> MADFLNFPRQMLPFSKKTKQWRKDCLLWANQKTFFNYSLVRKSVIHKKINYDLLNGRLHMSDLELVLNPDGIKAAYIPDRLQHYPIMNSKLNVLRGEESKRVFDFKVVVTNPNAISEIEDNKKNELLQRLQEMITDTSISEDEYNIKLEKLNDYYTYEWQDIREVRANELLNHYIKEYDIPLIFNNGFMDAMTCGEEIYQCDIVGGEPVIERVNPLKIRIFKSGYSNKVEDADMIILEDYWSPGRVIDTYYDVLSPKDIKYIETMPDYIGQGAVDQMDNIDERYGFVNQNMIGDEITVRDGTYFFDPANLFTEGIANSLLPYDLAGNLRVLRLYWKSKRKILKVKSYDPETGEEEWNFYPENYVVNKEAGEEVQSFWVNEAWEGTMIGNEIFVNMRPRLIQYNRLNNPSRCHFGIVGSIYNLNDSRPFSLVDMMKPYNYLYDAIHDRLNKAIASNWGSILELDLSKVPKGWDVGKWMYYARVNHIAVIDSFKEGTIGASTGKLAGALNNAGKGMIETNIGNYIQQQINLLEFIKMEMADVAGISKQREGQISQRETVGGVERATLQSSHITEWLFTIHDDVKKRALECFLETAKVALKGRNKKFQYILSDTSTRVMEIDGDEFAEADYGLVVDNSNGTQELQQKLDTLAQAALQTQTLSFSTITKLYTSSSLAEKQRLIEKDEKQIRERQAQAQKEQLEAQQQIAAMQQQQKEAELLQKEEANIRDNQTKIIIAQIQSEGGPDEEDGIMIDDYSPEAKANLAEKIREFDEKLKLDKDKLKLDKKKAETDASIKRQALRKKSSTT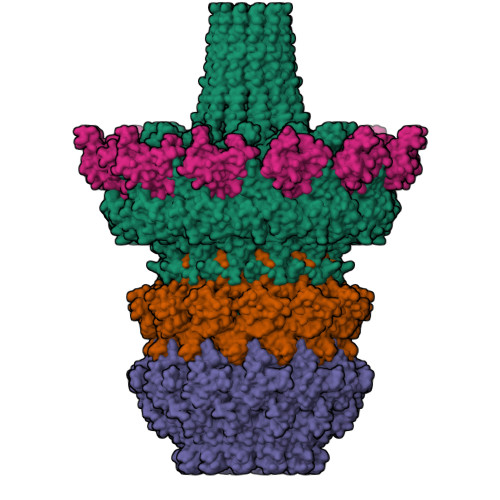NK;> MVNNINWVKLPVILDRLLRHPLLTDLNLETAIQYTLDFISAMGLPNVYVDKIETIDIKEYRGELPCDLISINQVRLHKNGIALRAMTDNFNAYPTHDHKEGDWYERGEPSFKTQGRVIFTSIKHEKVDISYKAIMLDDEGLPLIPDNPIFLKTLELYIKKEWFTILFDMGKISPAVLNNTQQEYAFKAGQCNNEFVIPSVSEMEAITNMWNQLIPRVTEFRRGFKNLGDKEYIRVH;> MTYNELIYMVLDELKLSSDDSYYTPDHVIFLLVKYRSFLLKQRYSDIKKQIPDSDYQSICLDLIEVPAISGEPCEGSSYLRSKNKVPTTMMIGNPRVYPMDFYQGEITYISRDRMRYVGYNKFLRNIIYCSKAPDGYLYFKSWNPQFLHLEKVSFNAIFEDAKEASEMACPEENGTICKLEDKEFPIEDALVPPLIELVVKELRGPEYSPKDEDNNAKDDLPDAR;>[2x]MAKKKIKRRGKMPPNIFDTGGQSWGQQSSGQFSNAFKGENLGNSIGSIGGAVGGIAQAGISNAQIADTSGIEAQNKAQKNMVVGASSNDDLMSEWGSWNKVKDDYSWKDVRGGSTGQRVTNTIGAAGQGAAAGASVGGPIGAIVGGVVGLGSAIGGWLGGNRKAKRKAKKLNKEAKEANERALTSFETRADNIDTQNDFNMLANFSAYGGPLEFGSGAIGYEFDNRYLNNQEMSAVAKQRLTSLPNSFQALPEMNTYNAFAEGGGLSREKNYGSKKKPYPSVPSGDFAGPHRSYPIPTKADARDALRLAGLHGNESVRRKVLAKYPSLKAFGGSLFDSVVGNNFNQSFTQGIQGMFQQEPEQTVQAANIAKDGGDIKIKEKNKGKFTAYCGGKVTEACIRKGKNSSNPTTRKRATFAQNARNWNAFGGWLNTQGGDFTNGVTFINEGGSHEENPYQGIQIGVDPEGAPNLVEQGEVVYDDYVFSDRMEIPDDIRKEYKLRGKTFAKAAKSAQRESEERPNDPLSTKGLQAAMERIATAQEEARQRKEAHREGNEYPSMFAYGGDTNPYGLALEDPMSVEELEALMVQSGETGEIAPEGNNGNRQTWTRYAPIIGSGLASLSDLFSKPDYDSADLISGVDLGAEAVGYAPIGNYLSYRPLDRDFYINKMNQQAAATRRGLMNTSGGNRLNAQAGILAADYNYGQNMGNLARQAEEYNQQLRERVEAFNRGTNMFNTETGLKASMFNAESRNAAKRARLGQATTVAQLRQGIKDQDAARRSANITNFLQGLGDMGWENEQANWLDTLAKSGVLKMNTKGEYTGGTKKAKGGKVRTKKKKGLTYG> GPGSNSKNPVPVKKEAKLSEAELHDKIKNLEEEKAELFEKLDKVEE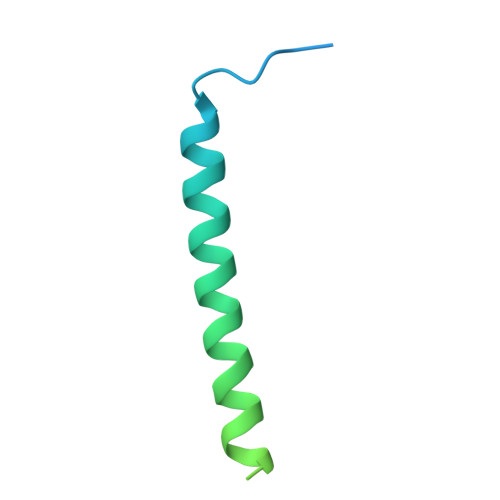EHKKVEEEHKKDHEKLEKKSEDVERHYLRQLDQEYKEQQERQKNLEELERQSQREVEKR> AEQISHKKSL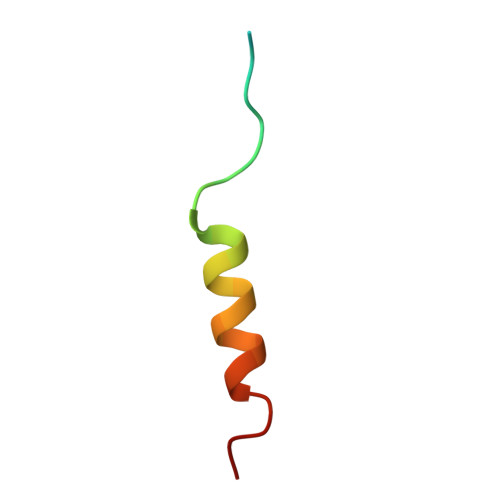RVSSLNKDRRLLLREFYNL>[15x]MKSLRKMLPALLILTPLLFSPAAAEEFSASFKGTDIQEFINTVSKNLNKTVIIDPSVRGTITVRSYDMLNEEQYYQFFLSVLDVYGFAVINMNNGVLKVVRAKDAKTSAVPVASAAAPGEGDEVVTRVVPLTNVAARDLAPLLRQLNDNAGAGSVVHYEPSNVLLMTGRAAVIKRLLTIVERVDNAGDRSVVTVPLSWASAAEVVKLVTELNKDTSKSALP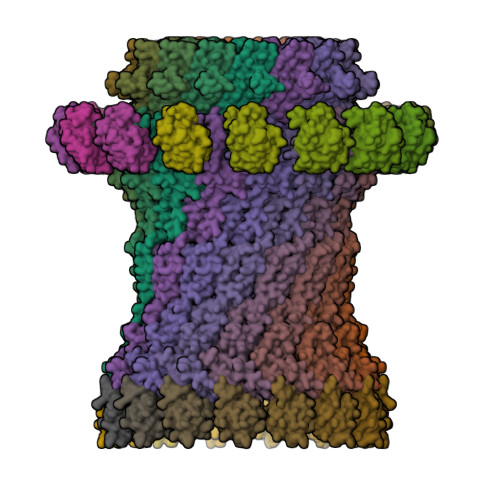GSMVANVVADERTNAVLVSGEPNSRQRIIAMIKQLDRQQAVQGNTKVIYLKYAKAADLVEVLTGISSSLQSDKQSARPVAAIDKNIIIKAHGQTNALIVTAAPDVMNDLERVIAQLDIRRPQVLVEAIIAEVQDADGLNLGIQWANKNAGMTQFTNSGLPISTAIAGANQYNKDGTISSSLASALGSFNGIAAGFYQGNWAMLLTALSSSTKNDILATPSIVTLDNMQATFNVGQEVPVLTGSQTTSGDNIFNTVERKTVGIKLKVKPQINEGDAVLLEIEQEVSSVADSASSTSSDLGATFNTRTVNNAVLVGSGETVVVGGLLDKTVTDTADKVPLLGDIPVIGALFRSDSKKVSKRNLMLFIRPTIIRDRDEYRQASSGQYTAFNNAQTKQRGKESSEASLSNDLLHIYPQQETQAFRQVSAAIDAFNLGGRP;>[15x]MIHYFDYSMMRIPLIFPLCMVALLSGCQQKPASTLSPAISSQAQLEQLSSVAAGTRYLKNKCNRSDLPADETIYRAAVNVGKARGWGNIDVATLSQNSDRLYQQLLQDSTPEATQCSQFNRQLAPFIASLRSDGSDYKDDDDK;>MPVSVMRLTNINKGIIKLLPQIVTLIILITAIPQLAKLTWRVVFPVSPEDISALPLTMPPAADPELKNVRPAFTLFGLAVKNSPTPTDAASLNQVPVSSLKLRLAGLLASSNPARSIAIIEKGNQQVSLSTGDPLPGYDARIAAILPDRIIVNYQGRKEAILLFNDSRAPSPPPTAAGNPPLVKRLREQPQNILTYLSISPVLSGDKLLGYRLNPGKDASLFRQSGLQANDLAIALNGIDLRDQEQAQQALQNLADMTEITLTVEREGQRHDIAFALGDE[15x]>[2x]MMWKIAVVDDDKNILKKVSEKLQQLGRVKTFLTGEDFLNDEEAFHVVV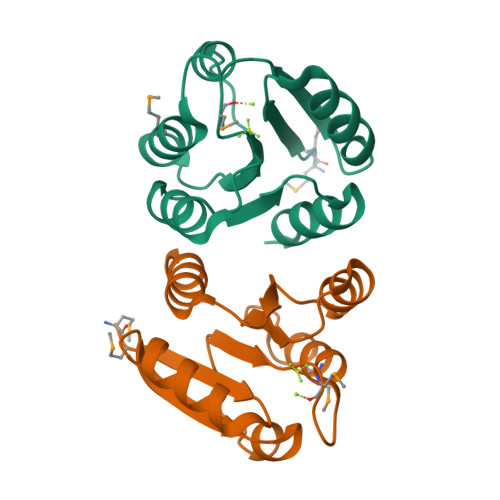LDVMLPDYSGYEICRMIKETRPETWVILLTLLSDDESVLKGFEAGADDYVTKPFNPEILLARVKRFLER>[4x]MDVSFRLSGATSSSYGVFISNLRKALPYERKLYDIPLLRSTLPGSQRYALIHLTNYADETISV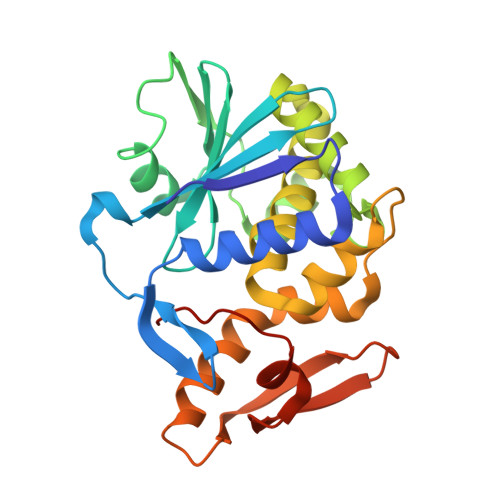AIDVTNVYVMGYRAGDTSYFFNEASATEAAKYVFKDAKRKVTLPYSGNYERLQIAAGKIRENIPLGLPALDSAITTLFYYNANSAASALMVLIQSTSEAARYKFIEQQIGKRVDKTFLPSLAIISLENSWSALSKQIQIASTNNGQFETPVVLINAQNQRVTITNVDAGVVTSNIALLPNRNNMA> MGSSHHHHHHSQDPKPRCAATKANDHNQAAFGRQWQGRGIYKGRDSWSNIMLKEGDIVYGGAPGQSGFYFNKATLDAAGGSR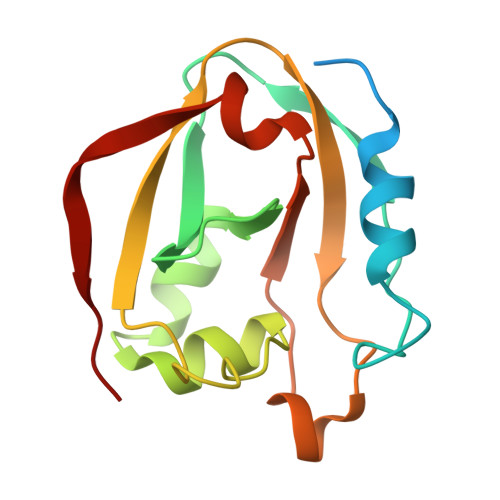AKLWESLQVLPHEKFGYRSKIQAYRVKRETIAGTGKAISQDPTRFGEGGGTQFFLSNYKTVLEPIDKPFEIGL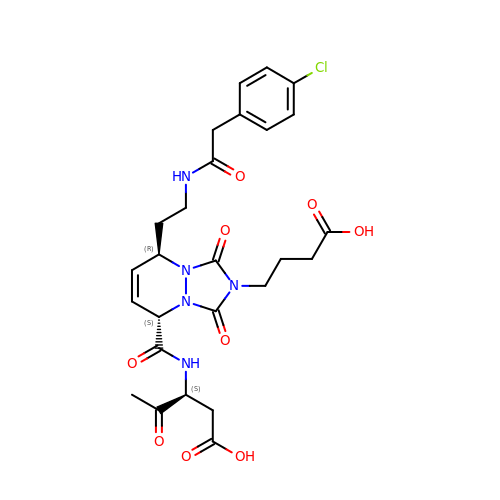(3S)-3-({[(5S,8R)-2-(3-carboxypropyl)-8-(2-{[(4-chlorophenyl)acetyl]amino}ethyl)-1,3-dioxo-2,3,5,8-tetrahydro-1H-[1,2,4]triazolo[1,2-a]pyridazin-5-yl]carbonyl}amino)-4-oxopentanoic acid | C26 H30 Cl N5 O9 | FCUBCMCZKNHBIS-UFYCRDLUSA-N> GSPAKIKIVAPLESALIPGGETYQLRCDIMSTPAATIHWKFNGKLIQGSNELNVEEKLLNFGKAIVDTGIVASILTIQCPSAENSGTYSCVGYNGHQTIETVAEVEIEGEASGCRSNHKSAPEIVFWTDSRFEMTGNVATLVCRANQQVDWVWMSNDELVKNNDKFTVLSNGDLVIKNIVWDDMGTYTCIARNQFGEARQETFLYPTAHHHHHH;> VPAPGETRACGRKLISLVMAVCGDLCNPQ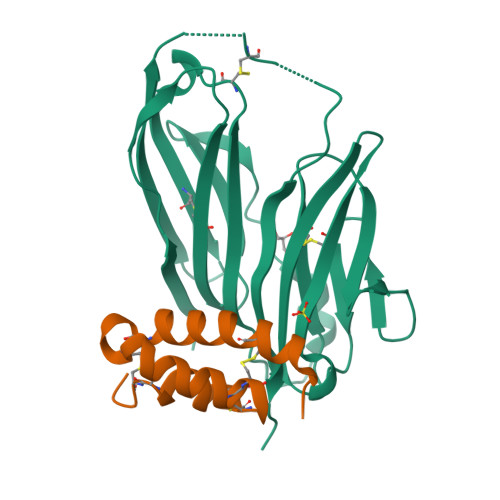EGKDIATECCGNQCSDDYIRSACCPHHHHHH cyclical inhibitor OD36 | C16 H15 Cl N4 O2 | 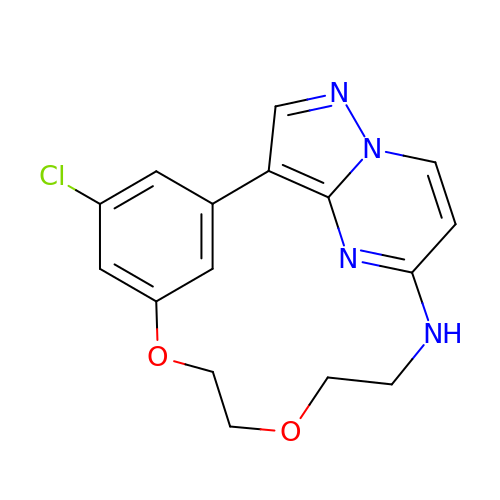KTSDBMVHAKWDRK-UHFFFAOYSA-N> HNHNHNHNHNHNGGENLYFQGASLTEIEHLVQSVCKSYRETCQLRLEDLLRQRSNIFSREEVTGYQRKSMWEMWERCAHHLTEAIQYVVEFAKRLSGFMELCQNDQIVLLKAGAMEVVLVRMCRAYNADNRTVFFEGKYGGMELFRALGCSELIS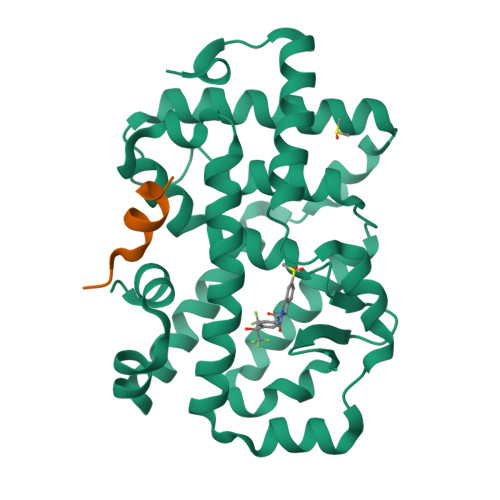SIFDFSHSLSALHFSEDEIALYTALVLINAHRPGLQEKRKVEQLQYNLELAFHHHLCKTHRQSILAKLPPKGKLRSLCSQHVERLQIFQHLHPIVVQAAFPPLYKELFSGG;> GKEKHKILHRLLQDSS> HPTFNKITPNLAEFAFSLYRQLAHQSNSTNIFFSPVSIATAFAMLSLGTKADTHDEILEGLNFNLTEIPEAQIHEGFQELLRTLNQPDSQLQLTTGNGLFLSEGLKLVDKFLEDVKKLYHSEAFTVNFGDTEEAKKQINDYVEKGTQGKIVDLVKELDRDTVFALVNYIFFKGKWERPFEVKDTEEEDFHVDQVTTVKVPMMKRLGMFNIQHCKKLSSWVLLMKYLGNATAIFFLPDEGKLQHLENELTHDIITKFLENEDRRSASLHLPKLSITGTYDLKSVLGQLGITKVFSNGADLSGVTEEAPLKLSKAVHKAVLTIDEKGTEAAGAMFL;> EAIPRSIPPE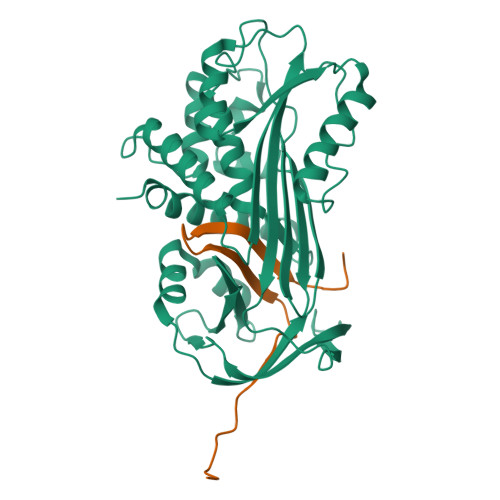VKFNKPFVFLMIEQNTKSPLFMGKVVNPTQK>MHHHHHHMAHFMDVHRGMHGITSDQLHQAHQADLAVEKDENVHFEQAWADPASGTIYCLSEGPSAEAVQRVHERAGHKADEIHEV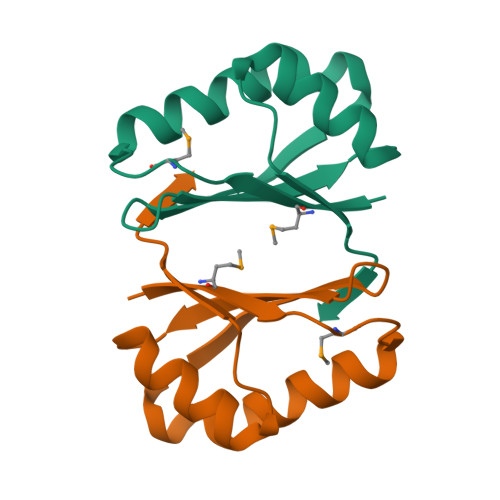PLSA[2x]Human Epidermal growth factor Receptor 4 (HER4 or ERBB4) carries out essential functions in the development and maintenance of the cardiovascular and nervous systems. HER4 activation is regulated by a diverse group of extracellular ligands including the neuregulin (NRG) family and betacellulin (BTC), which promote HER4 homodimerization or heterodimerization with other HER receptors. Important cardiovascular functions of HER4 are exerted via heterodimerization with its close homolog and orphan receptor, HER2. Here, we report cryo-EM structures of near full-length HER2/HER4 heterodimers and full-length HER4 homodimers bound to NRG1β and BTC.

To test this hypothesis for HER4 complexes, we determined the cryo-EM structures of full-length HER4 homodimers bound to NRG1β or BTC. In both structures, HER4 kinase domains were bound to afatinib to enable high-resolution reconstruction in the ECD module (3.4 Å for NRG1β, and 3.7 Å for BTC). As observed in a previous HER4/NRG1β crystal structure of isolated ECDs, liganded HER4 assembles into homodimers with near-perfect C2 symmetry. The two receptors in the HER4/NRG1β dimer adopt an angle of 37 degrees compared to 33 degrees for HER4/BTC. Detailed 3D classification analysis revealed substantial scissor-like movements around the dimerization arm in both data sets with the concerted intermonomer movement of domains I and IV, varying from 35 to 39 degrees for HER4/NRG1β and 30–35 degrees for HER4/BTC. While both pockets bury a similar surface area (NRG1β: 2967–3068 A2, BTC: 3142–3163 A2), the HER4/NRG1β pocket is characterized by a larger network of ionic interactions. In the HER4/NRG1β pocket, HER4 K438, K35, E112 and D376 form salt bridges with NRG1β E215, D219, R207 and R220, respectively. Most remarkably, at lower contour levels, our HER4 maps show continuous cryo-EM density connecting the two receptor monomers originating from N548 and N576 on domain IV of one receptor monomer and N358 on domain III of the other receptor involving sugar moieties beyond the core glycan trees of 4–5 sugars. Indeed, 3D classification of the particles in our final reconstruction uncovered at least one class with more defined N548-N576-N358 glycan networks in the dimer interface. Thus, our analysis of the HER4/NRG1β homodimer cryo-EM density uncovers an important role of receptor glycosylation in stabilizing the active HER4 monomer by bridging its two distal domains, domain II and IV and domains I and II, and likely both monomers within the HER4 homodimer through direct inter-receptor connections.

>[2x]QSVCAGTENKLSSLSDLEQQYRALRKYYENCEVVMGNLEITSIEHNRDLSFLRSVREVTGYVLVALNQFRYLPLENLRIIRGTKLYEDRYALAIFLNYRKDGNFGLQELGLKNLTEILNGGVYVDQNKFLCYADTIHWQDIVRNPWPSNLTLVSTNGSSGCGRCHKSCTGRCWGPTENHCQTLTRTVCAEQCDGRCYGPYVSDCCHRECAGGCSGPKDTDCFACMNFNDSGACVTQCPQTFVYNPTTFQLEHNFNAKYTYGAFCVKKCPHNFVVDSSSCVRACPSSKMEVEENGIKMCKPCTDICPKACDGIGTGSLMSAQTVDSSNIDKFINCTKINGNLIFLVTGIHGDPYNAIEAIDPEKLNVFRTVREITGFLNIQSWPPNMTDFSVFSNLVTIGGRVLYSGLSLLILKQQGITSLQFQSLKEISAGNIYITDNSNLCYYHTINWTTLFSTINQRIVIRDNRKAENCTAEGMVCNHLCSSDGCWGPGPDQCLSCRRFSRGRICIESCNLYDGEFREFENGSICVECDPQCEKMEDGLLTCHGPGPDNCTKCSHFKDGPNCVEKCPDGLQGANSFIFKYADPDRECHPCHPNCTQGCNGPTSHDCIY;>[2x]SHLVKCAEKEKTFCVNGGECFMVKDLSNPSRYLCKCPNEFTGDRCQNYVMAS>MSAIENFDAHTPMMQQYLRLKAQHPEILLFYRMGDFYELFYDDAKRASQLLDISLTKRGASAGEPIPMAGIPYHAVENYLAKLVNQGESVAICEQIGDPATSKGPVERKVVRIVTPGTISDEALLQERQDNLLAAIWQDSKGFGYATLDISSGRFRLSEPADRETMAAELQRTNPAELLYAEDFAEMSLIEGRRGLRRRPLWEFEIDTARQQLNLQFGTRDLVGFGVENAPRGLCAAGCLLQYAKDTQRTTLPHIRSITMEREQDSIIMDAATRRNLEITQNLAGGAENTLASVLDCTVTPMGSRMLKRWLHMPVRDTRVLLERQQTIGALQDFTAGLQPVLRQVGDLERILARLALRTARPRDLARMRHAFQQLPELRAQLETVDSAPVQALREKMGEFAELRDLLERAIIDTPPVLVRDGGVIASGYNEELDEWRALADGATDYLERLEVRERERTGLDTLKVGFNAVHGYYIQISRGQSHLAPINYMRRQTLKNAERYIIPELKEYEDKVLTSKGKALALEKQLYEELFDLLLPHLEALQQSASALAELDVLVNLAERAYTLNYTCPTFIDKPGIRITEGRHPVVEQVLNEPFIANPLNLSPQRRMLIITGPNMGGKSTYMRQTALIALMAYIGSYVPAQKVEIGPIDRIFTRVGAADDLA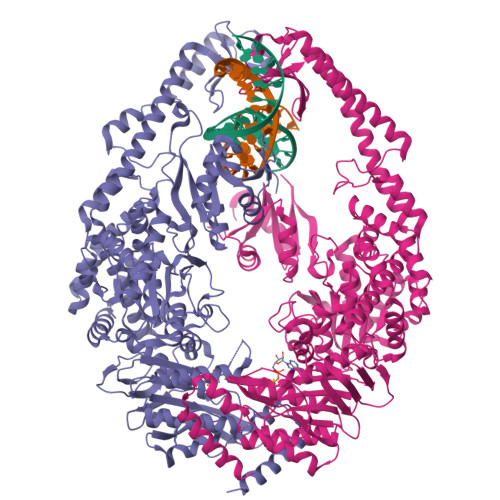SGRSTFMVEMTETANILHNATEYSLVLMDEIGAGTSTYDGLSLAWACAENLANKIKALTLFATHYFELTQLPEKMEGVANVHLDALEHGDTIAFMHSVQDGAASKSYGLAVAALAGVPKEVIKRARQKLRELESIS[2x]> MEILRYLMDPDTFTSNFNNDPLVLRRRQTYLCYEVERLDNGTSVKMDQHMGFLCNESGRHAELRFLDLVPSLQLDPAQIYRVTWFISWSPCFSWGCAGEVRAFLQENTHVRLRIKAARIYDDQGRCQEALQMLRDAGAQVS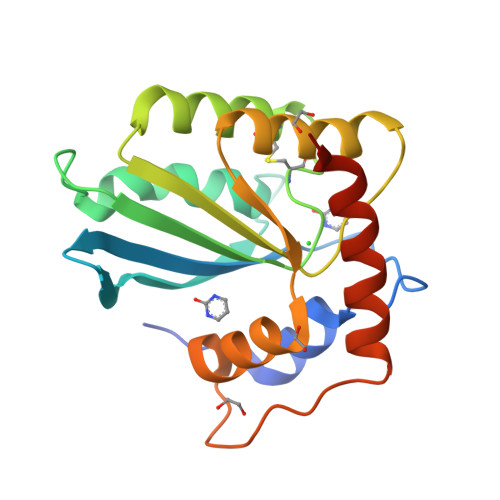IMTYDEFEYCWDTFVYRQGCPFQPWDGLEEHSQALSGRLRAILQLEHHHHHH> MELMMAIGYLGLALVLGSLVAKIAEKLKIPDIPLLLLLGLIIGPFLQIIPSDSAMEIFEYAG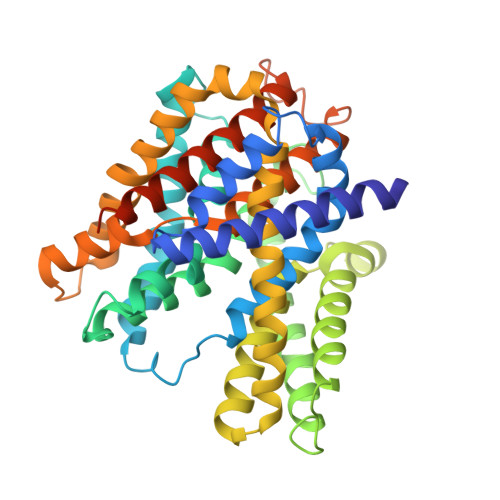PIGLIFILLGGAFTMRISLLKRVIKTVVRLDTITFLITLLISGFIFNMVLNLPYTSPVGYLFGAITAATDPATLIPVFSRVRTNPEVAITLEAESIFNDPLGIVSTSVILGLFGLFSSSNPLIDLITLAGGAIVVGLLLAKIYEKIIIHCDFHEYVAPLVLGGAMLLLYVGDDLLPSICGYGFSGYMAVAIMGLYLGDALFRADDIDYKYIVSFCDDLSLLARVFIFVFLGACIKLSMLENYFIPGLLVALGSIFLARPLGVFLGLIGSKHSFKEKLYFALEGPRGVVPAALAVTVGIEILKNAEKIPASITKYITPTDIAGTIIIGTFMTILLSVILEASWAGMLALKLLGEYKPKYKEESHH>GAMGSGIQPNVNEYMFSNKFKARVMVSRKAPEGVTVNDTYDHKEDILKYEWFEFILPEGNFSATMTIDLMNNAIIDNYLEIGRQNGVLESDIGVKFDTRNFRLGWDPETKLIMPGVYTYEAFHPDIVLLPGCGVDFTESRLSNLLGIRKRHPFQEGFKIMYEDLEGGNIPALLDVTAYEESKKDTTTETTTKKELKIQPLEKDSKSRSYNVLEDKINTAYRSWYLSYNYGNPEKGIRSWTLLTTSDVTCGANGDSGNPVFSKSFYNEQAVYSQQLRQATSLTHVFNRFPENQILIRPPAPTITTVSENVP[5x]

Adenovirus-derived nanoparticles (ADDomer) comprise 60 copies of adenovirus penton base protein (PBP). In the ADDomer, the PBP monomers spontaneously assembles to form a pentamer, and twelve pentamers organize into a dodecamer characterized by high stability and thermotolerance exceeding 50°C.16–18 The PBP monomer folds into two distinctive domains; the jelly-roll fold domain which is located in the core of the dodecamer and assumed to be responsible for multimerization, and a solvent-facing exterior domain, called the crown domain. The crown domain comprises two highly flexible regions, called variable loop (VL) and arginine-glycine-aspartic acid (RGD) motif-containing loop. To expand the scope of ADDomers for new applications, we engineered ADDobodies, representing PBP crown domain, genetically separated from PBP multimerization domain.

To validate our design by high-resolution structural analysis using X-ray crystallography, we created an ADDobody prototype with minimized loops, called ADDobody-Xtal, based on the assumption that long flexible loops could be detrimental to crystal lattice formation. ADDobody with minimized VL and RGD loop sizes (ADDobodyXtal) was crystallized. Crystals grew under two different conditions, one containing 0.1 M zinc acetate and the other devoid of zinc. ADDobody crystals grown in the presence of zinc adopted space group P212121, and diffracted to a resolution of 2.90 Å. The crystallization of ADDobody proteins in the presence of zinc resulted in crystals with a characteristic needle-like shape. In this zinc-containing crystal form, ADDobodies also adopted a pentamer; however, the pentameric rings are not stacked on top of each other. Rather, a zinc ion mediates the interaction between pentamer rings participating in crystal packing. The zinc ion is coordinated by four residues from four different ADDobody chains: H151 donated from one chain, E13 from an adjacent ADDobody chain of the same pentamer, and H151 and E13 from the juxtaposed pentameric ring. The RGD loop region clearly lacked density for about 12−15 residues in all chains of both refined structures indicating conformational disorder. Moreover, the structures imply that multimerization on the level of the pentamer in the ADDomer nanoparticle may not be mediated by the jelly-roll fold domains alone, but that the crown domains also contribute, given that the ADDobodies were found to form pentameric rings in both crystal forms, in spite of being monomeric in solution.>MSDQKTVHDVTYDLLRKLGLTTVFGNPGSTEESFLRDFPEDFTYVLSLQEASALAMADGFAQATGKPALVNLHTAAGTGNAMGSLVAAYRANTPLIITAGQQTREMSVVDPYLNNPDATTMPKPWVKWSYEPARAEDVPAAFMQAYAVAMQPPMGPVFLSIPLDDWDKPALGPAAVRSVSTRVAPDAERLAQFAERINAAKHPMLVLGPEVDRAGAWDAGIEFAEKLGAPVHASALPDRMSFPEDHPLYAGPLPMTIAGVEQAVSAYDLVVVVGAEVFRYYPYVPGEYLPEGTDLLQITADPHRSAVAPVGDSLVGDVGIALSRLTELIDTPDDRV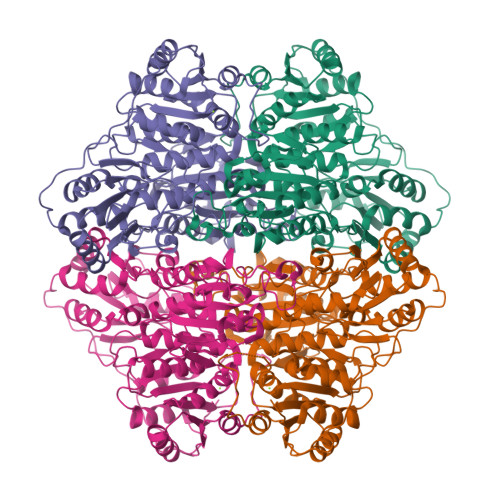PPKPLVRQRHSDIPSTAPMTSNAVYEVLSNVKPDDAAVVMESTSTMLDLFTWLPTTHPASFFATGSGGIGWGVPAAVGIALGDRARGVDRTVVATIGDGSFQYSIQAIWTAAQHKLPIVFVVLRNGEYAILKSFADLEKTPNVPGLQLPGLDISSIAAGFGCRTATVESTDMLEAELKTALQADGPTVLVVPTLPQLPQLGRSHHHHHH[2x]> SAQLLKSVFVKNVGWATQLTSGAVWVQFNDGSQLVVQAGVSSISYTSPNGQTTRYGENEKLPDYIKQKLQCLSSILLMFSNPTPNFH;> PDAYRFLTEQDRQLRLLQAQIQ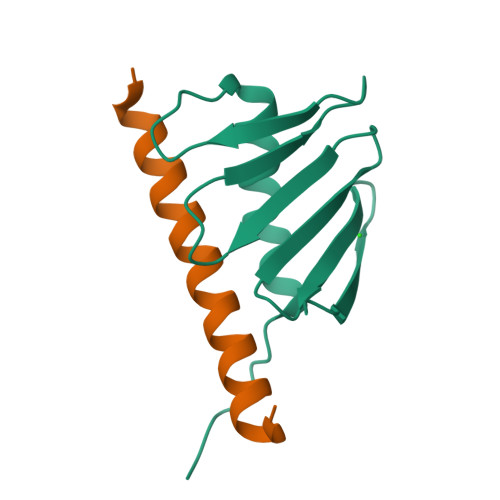RLLEAQSLMP PARA-(BENZOYL)-PHENYLALANINE | C16 H15 N O3 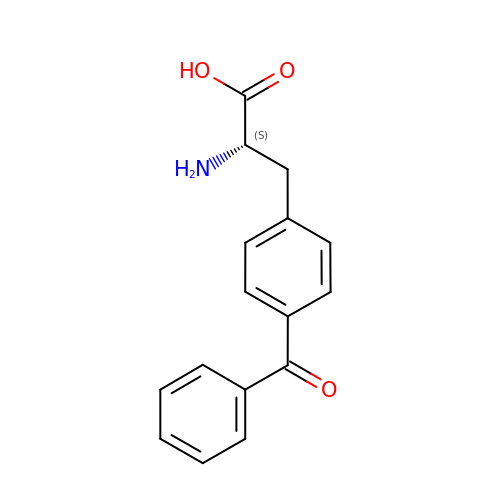| TVIDEEHSOPHZBR-AWEZNQCLSA-N>DCPSGWSSYEGNCYKFFQQKMNWADAERFCSEQAKGGHLVSIKIYSKEKDFVGDLVTKNIQSSDLYAWIGLRVENKEKQCSSEWSDGSSVS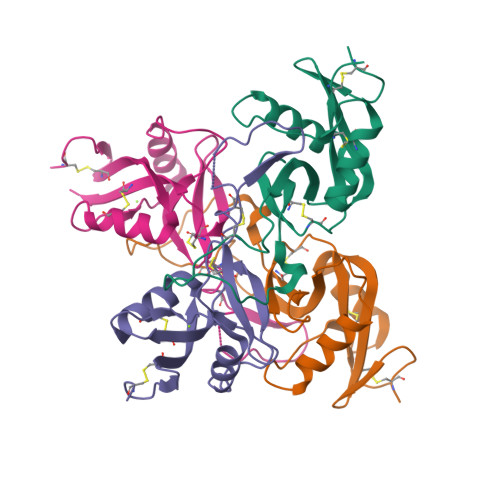YENVVERTVKKCFALEKDLGFVLWINLYCAQKNPFVCKSPPP[2x];>DCPPDWSSYEGHCYRFFKEWMHWDDAEEFCTEQQTGAHLVSFQSKEEADFVRSLTSEMLKGDVVWIGLSDVWNKCRFEWTDGMEFDYDDYYLIAEYECVASKPTNNKWWIIPCTRFKNFVCEFQA[2x]>GAMLSTLPVPPSQRDNLEASFAIVSAEECDPTDDICEIGVRMEEQLAKQLMMCKNTRDHHKAMGDVAGMNRFENLALTVQKDLDLVRYSKRKNEPLPKFHYEKRSFNIVHCNTDLTDSELEIVVVRGISYNVANPKDVDTYVRVEFPLLNDESFKTKTNVIRDTSSPDYDERFKVDIQRTNRQFQRIFKRHGVKFEIYSRGGFLRSDTLIGTVNVKLQPLETKCEIHDTYDLMDGRKQVGGKLEVKIRVRNPILTKQMEHITEKWLVLDA[2x]

In this work, we have explored the function of coiled-coil- and C2 domain-containing protein B (CC2D1B), a poorly characterized member of the Lgd/CC2D1 family of proteins that also includes the closely related human CC2D1A and its D. melanogaster ortholog Lgd. These proteins are characterized by the presence of four tandem DM14 domains that interact with the CHMP4 family of ESCRT-III proteins (Martinelli et al., 2012, Troost et al., 2012, Usami et al., 2012) and one C-terminal C2 domain that mediates their binding to membrane lipids (Drusenheimer et al., 2015, Gallagher and Knoblich, 2006). Therefore, we reveal CC2D1B as an essential regulatory factor that licenses the formation of ESCRT-III polymers to ensure the orderly reformation of the NE.

We then explored functional determinants shared by the Lgd/CC2D1 family, thereby performing structural studies of the highly conserved C-terminal region of the Drosophila ortholog Lgd. The structure revealed an α-helical N-terminal domain that contains a ∼50 Å long helical hairpin, followed by a long coil structure arranged anti-parallel to the hairpin which connects to the C2 domain at amino acid 664. The C2 fold ends at amino acid 796 and the remaining C-terminal region (residues 797–815) intertwines with the N-terminal helical domain, thereby stabilizing it. The C2 domain of Lgd forms a classical β-sandwich structure with two four-stranded β sheets that classifies as a class II C2 domain with N and C termini oriented at the bottom of the sandwich and opposite to the top loops, similar to the topology of the phospholipase C-δ1 C2 domain (Essen et al., 1996). The Lgd C2 domain is atypical as two short α helices are inserted into the loops connecting β strands 5 with 6 (α3) and β- 7 with 8 (η2). These α helices are conserved in human CC2D1A/B orthologs, suggesting that these regions are functionally important. The convex part of the C2 domain is rigidly connected to the N-terminal α-helical domain via multiple interactions. Interestingly, this cluster is conserved in Lgd (residues R689, K701, K703) as well as in eukaryotic orthologs including human CC2D1B, which is consistent with the ability of CC2D1A and CC2D1B to associate with membrane pellets in cell fractioning experiments (Drusenheimer et al., 2015).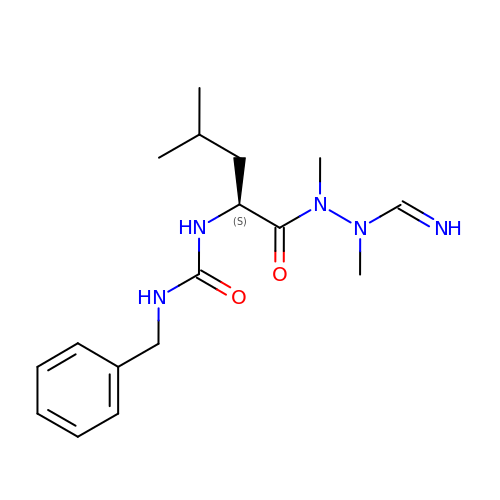1-[(2~{S})-1-[[iminomethyl(methyl)amino]-methyl-amino]-4-methyl-1-oxidanylidene-pentan-2-yl]-3-(phenylmethyl)urea | C17 H27 N5 O2 | DZXGVGCCLHWTMQ-BRYHAGSVSA-N>[2x]TSTMGNLQTAINDKSGTLASQNFLDADEQKRNAYNQAVSAAETILNKQTGPNTAKTAVEQALNNVNNAKHALNGTQNLNNAKQAAITAINGASDLNQKQKDA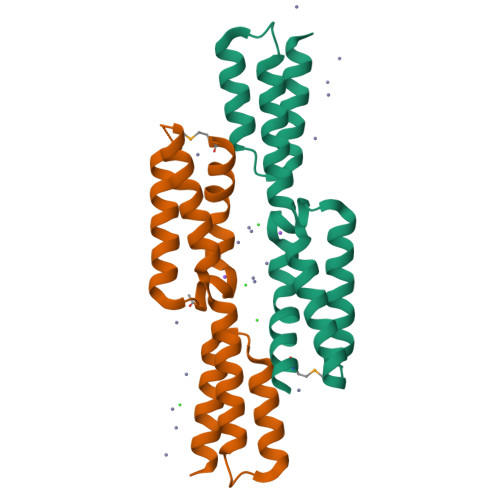LKAQANGAQRVSNAQDVQHNATELNTA methyl N-(2,3-dihydroxybenzoyl)-O-formyl-L-serinate 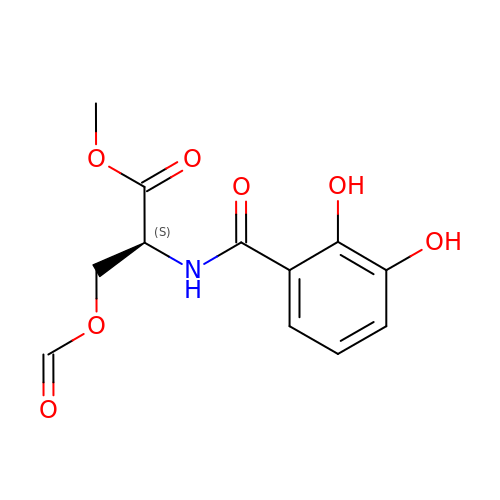| C12 H13 N O7 | SHACLOMOOCNGDP-QMMMGPOBSA-N Twinkle is a mitochondrial replicative helicase which can self-load onto and unwind mitochondrial DNA. The N-terminal domain (NTD) of Twinkle is derived from the TOPPRIM family primase. The helicase domain is located on the C-terminal half of Twinkle. Similar to gp4 and DnaB, Twinkle forms a homo-hexamer and migrates in the 5′ to 3′ direction on the single-stranded DNA (ssDNA).

Thus, the purified E325Q LcTwinkle–DNA–ATP complex from gel filtration was used for cryo-EM analysis. We determined the LcTwinkle–DNA complex structure with cryo-EM at 3.5 Å resolution. LcTwinkle forms a homo-hexamer wrapping DNA in its central channel. The CTDs form a non-planar lock-washer-shaped hexamer, similar to gp4 and DnaB. The NTDs are attached to the side of the CTDs. An extended linker connects the NTD and the CTD (N–C linker) in a domain-swapped manner. ATPase sites are located at each of the subunit interfaces, and five ATP molecules can be refined. A 12 nt ssDNA binds to the central channel of LcTwinkle, with an average of 2 nt per subunit. The almost identical configurations of the ATP-binding sites in the LcTwinkle hexamer suggested that all subunits have a similar chance of hydrolyzing ATP. The domain-swapped interface is a hotspot for disease-related mutations.

>[6x]MQKEEQDFLSPHVMLGYPESLDEQEEGERELREVQRIWSSAVPFNDLPEDEAQLIKTMFQITKVSNATLKKFGVRLFKPTKSLVFPWFAGPDSSLKGLKLLSAQNTDTEKVTYNEATVPKISSYYNLFGLTLVGRMDSEVVLTGHELDTLAVSQATGLPSVALPRGVSCLPPMLLPYLEQFKRVTLWLGHDIRSWEASKIFSRKLGLRRCSLVRPGEDRPCPLEALARGKNLSRIIKTSIPAAHKSIVSFKQLREDVYGELLNTEQVAGVKWTRFPELNRILKGHRKGELTVFTGPTGSGKTTFISEVALDLCIQGVNTLWGSFQINNVRLAKIMLTQFAMQRLEENLEQYDFWADKFEELPLYFMTFHGQQNIKTVLDTMQHAVYLYDINHVIIDNLQFMMGQENLSIDKYAVQDHIIGAFRKFATNTSCHVTLIIHPRKEEDDRELQTASIFGSAKASQEADNVLILQEKKLVTCPGRRSLQVTKNRFDGDVGIFPLDFIKSSLTFSAPIKGKVKLRKVSTKPENEEVGGERGGSEEGRG> GSHMRLDKFIAQQLGVSRAIAGREIRGNRVTVDGEIVRNAAFKLLPEHDVAYDGNPLAQQHGPRYFMLNKPQGYVCSTDDPDHPTVLYFLDEPVAWKLHAAGRLDIDTTGLVLMTDDGQWSH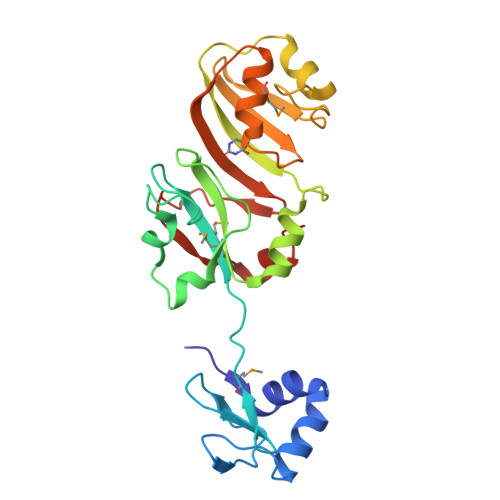RITSPRHHCEKTYLVTLESPVADDTAEQFAKGVQLHNEKDLTKPAVLEVITPTQVRLTISEGRYHQVKRMFAAVGNHVVELHRERIGGITLDADLAPGEYRPLTEEEIASVV> MAKIGLF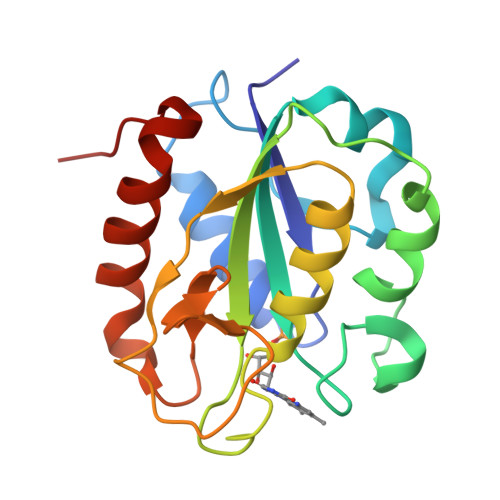FGSDTGTTRKIAKQIKDMFDDEVMAKPLNVNRADVADFMAYDFLILGTPTLGDGQLPGLSANAASESWEEFLPRIADQDFSGKTIALFGLGDQVTYPLEFVNALFFLHEFFSDRGANVVGRWPAKGYGFEDSLAVVEGEFLGLALDQDNQAALTPERLKGWLSLIAADFGLVLPA>GPEKGERISMINPRVVLDENGISHRSRYFIMLCDNETAIAHAKKTSIWAVKKDSSKRISDAYKKASVYFIFVAQQTYNALGYAQVVSDLNSTELPFWSDSSHAGGVRIKWIKTCNLFSAEISEIVSHMDHGSEARDGMEMMYDEGSRLCTLINYAIMKRIGRDR[2x]

Mmi1 is an essential RNA-binding protein in the fission yeast Schizosaccharomyces pombe that eliminates meiotic transcripts during normal vegetative growth. A C-terminal YTH RNA-binding domain in Mmi1 recognizes UNAAAC motifs (where N is any ribonucleotide) that are present in multiple copies within DSRs. Surprisingly, Mmi1 binds DSR RNA using a divergent mechanism on a surface that is distinct from the m6A-binding pocket, including extended protein sequences located upstream and downstream of the YTH domain. We propose that the low-complexity region influences RNA binding indirectly by reducing dynamic motions of the RNA-binding groove and stabilizing a conformation of the YTH domain that binds to RNA with high affinity.

We also determined a structure of apo-Mmi1 residues 327–488. The core YTH domain of our structure of Mmi1-RNA is similar to apo-Mmi1 and to previously reported structures with a central five-stranded β-sheet surrounded by four α-helices. Interestingly, the low-complexity N-clamp region adopted a similar conformation in two structures of Mmi1 determined in the absence of RNA (this work and Ref. 21). Both apo- and RNA-bound structures have crystal-packing contacts in their N-terminal regions. Furthermore, structural alignments of all known Mmi1 YTH domain structures show that the core fold is highly similar (r.m.s.d. <0.5 Å), but the N- and C-clamps are more divergent. This observation is also consistent with higher relative B-factors in these regions.>GTGYTVGDFMTPRQNLHVVKPSTSVDDALELLVEKKVTGLPVIDDNWTLVGVVSDYDLLALDSISGRSQ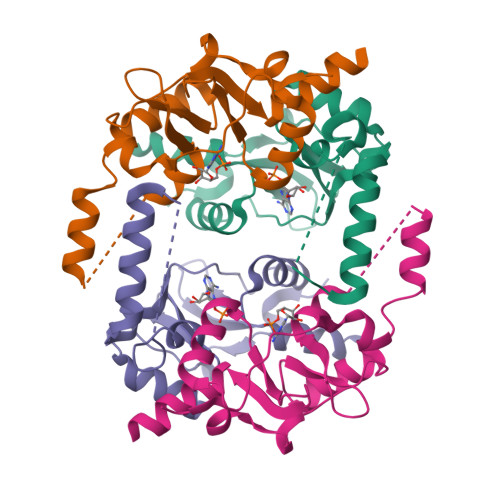NDTNLFPDVDSTWKTFNELQKLISKTYGKVVGDLMTPSPLVVRDSTNLEDAARLLLETKFRRLPVVDADGKLIGILTRGNVVRAALQIKRETENST[4x]> HHHHHHMKFTVEREHLLKPLQQVSGPLGGRPTLPILGNLLLQVADGTLSLTGTDLEMEMVARVALVQPHEPGATTVPARKFFDICRGLPEGAEIAVQLEGERMLVRSGRSRFSLSTLPAADFPNLDDWQSEVEFTLPQATMKRLIEATQFSMAHQDVRYYLNGMLFETEGEELRTVATDGHRLAVCSMPIGQSLPSHSVIVPRKGVIELMRMLDGGDNPLRVQIGSN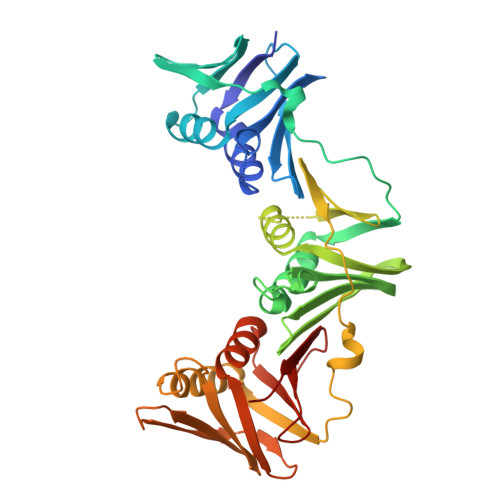NIRAHVGDFIFTSKLVDGRFPDYRRVLPKNPDKHLEAGCDLLKQAFARAAILSNEKFRGVRLYVSENQLKITANNPEQEEAEEILDVTYSGAEMEIGFNVSYVLDVLNALKCENVRMMLTDSVSSVQIEDAASQSAAYVVMPMRL> MFKLKLLSISTIFILAGCVSLAPEYQRPPAPVPQQFSLSKNSLTPAVNSYQDTGWRNFFVDPQVSRLIGEALNN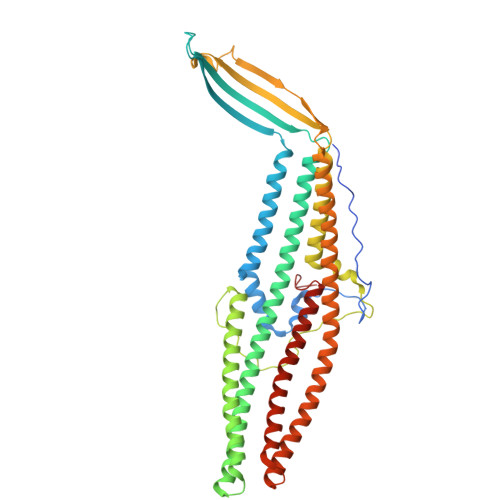NRDLRMAALKVEEARAQFNVTDADRYPQLNASSGITYNGGLKGDKPTTQEYDAGLELSYELDFFGKLKNMSEADRQNYFASEEARRAVHILLVSNVSQSYFSQQLAYEQLRIARETLKNYEQSYAFVEQQLVTGSTNVLALEQARGQIESTRAEIAKREGDLAQANNALQLVLGTYRAVPSEKGIKGGEIAPVKLPPNLSSQILLQRPDIMEAEYQLKAADANIGAARAAFFPSITLTSGLSSSSTELSSLFTSGSGMWNFIPKIEIPIFNAGRNKANLKLAEIRQQQSVVNYEQKIQSAFKDVSDTLALRDSLSQQLESQQRYLDSLQITLQRARGLYASGAVSYIEVLDAERSLFATQQTILDLTYSRQVNEINLFTALGGGWVEKH>[4x]MNVLFTSVPQEDVPFYQEALKDLSLKIYTTDVSKVPENELKKAELISVFVYDKLTEELLSKMPRLKLIHTRSVGFDHIDLDYCKKKGILVTHIPAYSPESVAEHTFAMILTLVKRLKRIEDRVKKLNFSQDSEILARELNRLTLGVIGTG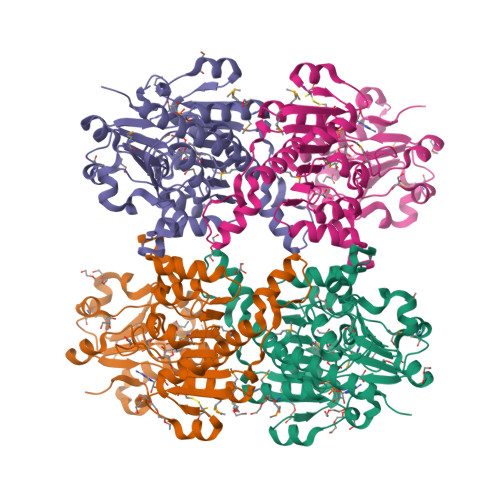RIGSRVAMYGLAFGMKVLCYDVVKREDLKEKGCVYTSLDELLKESDVISLHVPYTKETHHMINEERISLMKDGVYLINTARGKVVDTDALYRAYQRGKFSGLGLDVFEDEEILILKKYTEGKATDKNLKILELACKDNVIITPHIAYYTDKSLERIREETVKVVKAFVKGDLEQIKGNFVVGPS> 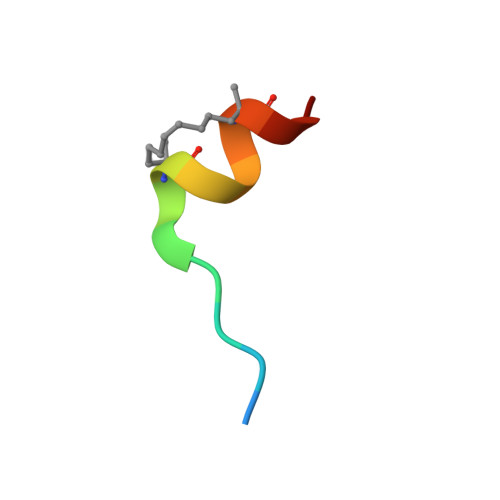XRIIYSRLQLLLLKX>[3x]QTQFTERALTILTLAQKLASDHQHPQLQPIHILAAFIETPEDGSVPYLQNLIEKGRYDYDLFKKVVNRNLVRIPQQQPAPAEITPSYALGKVLQDAAKIQKQQKDSFIAQDHILFALFNDSSIQQIFKEAQVDIEAIKQQALELRGNTRIDSRGADTNTPLEYLSKYAIDMTEQARQGKLDPVIGREEEIR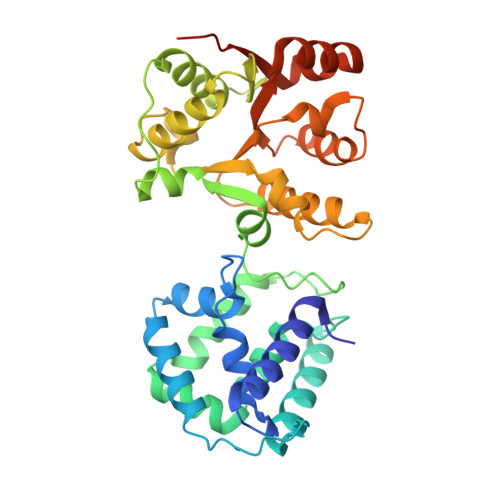STIRVLARRIKSNPCLIGEPGIGKTAIIEGVAQRIIDDDVPTILQGAKLFSLDLAALTAGAKYKGDFEERFKGVLKEIEESKTLIVLFIDEIHMLMGNGKDDAANILKPALSRGQLKVIGATTNNEYRSIVEKDGAFERRFQKIEVAEPSVRQTVAILRGLE>GGSRCQRDHLSTKLIPTEVPADLIRAVTCQVCDHLLSDPVQSPCRHLFCRLCIIRYTHALGPNCPTCNQHLNPSHLIKPAKFFLATLSSLPLLCPSEECSDWVRLDSFREHCLNHYREKESQEEQTPSEQNLDGYLPVNKGGRPRQHLLSLTRRAQKHRLRDLKNQVKTFAEKEEGGDVKSVCLTLFLLALRAGNEHKQADELEAMMQGRGFGLHPAVCLAIRVNTFLSCSQYHKMYRTVKATSGRQIFQPLHTLRNAEKELLPGFHQFEWQPALKNVSTSWDVGIIDGLSGWTVSVDDVPADTISRRFRYDVALVSALKDLEEDIMEGLRERALDDSMCTSGFTVVVKESCDGMGDVSEKHGSGPAVPEKAVRFSFTIMSISIRLEGEDDGITIFQEQKPNSELSCRPLCLMFVDESDHETLTAILGPVVAERKAMMESRLIISVGGLLRSFRFFFRGTGYDEKMVREMEGLEASGSTYICTLCDSTRAEASQNMVLHSITRSHDENLERYEIWRKNPFSESADELRDRVKGVSAKPFMETQPTLDALHCDIGNATEFYKIFQDEIGEVYQKPNPSREERRRWRSTLDKQLRKKMKLKPVMRMNGNYARRLMTREAVEAVCELVPSEERREALLKLMDLYLQMKPVWRSTCPSRDCPDQLCQYSYNSQQFADLLSSMFKYRYDGKITNYLHKTLAHVPEIVERDGSIGAWASEGNESGNKLFRRFRKMNARQSKTFELEDILKHHWLYTSKYLQKFMEAHKNS[2x];>GGSMSLQPLTAVNCGSLVQPGFSLLDLEGDVYLFGQKGWPKRSCPTGIFGVRIKKGELKLRAISFSNNSSYLPPLRCPAIAHFEAQDGKPECYLIHGGRTPNNELSSSLYMLSVDSRGCNRKVTLRCEEKELVGDVPSARYGHTLSVINSRGKTACVLFGGRSYMPPTERTTQNWNSVVDCPPQVYLIDLEFGCCTAHTLPELTDGQSFHVALARQDCVYFLGGHILSSDCRPSRLIRLHVELLLGSPVLTCTILHEGLTITSAIASPIGYHEYIIFGGYQSETQKRMECTYVGLDDVGVHMESREPPQWTSEISHSR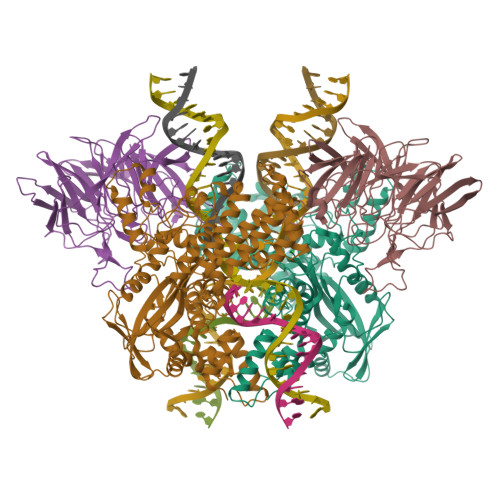TWFGGSLGKGTALVAIPSEGNPTPPEAYHFYQVSFQKEQDGEATAQGGSQESTDFEDSAPLEDSEELYFGREPHELEYSSDVEGDTYNEEDEEDESQTGYWIKCCLSCQVDPNIWEPYYSTELTRPAMIFCSRGEGGHWVHAQCMELPESLLLQLSQDNSKYFCLDHGGLPKQEMTPPKQMLPVKRVPMKMTHRKAPVSLKMTPAKKTFLRRLFD[2x]> MAPITAYSQQTRGLLGCI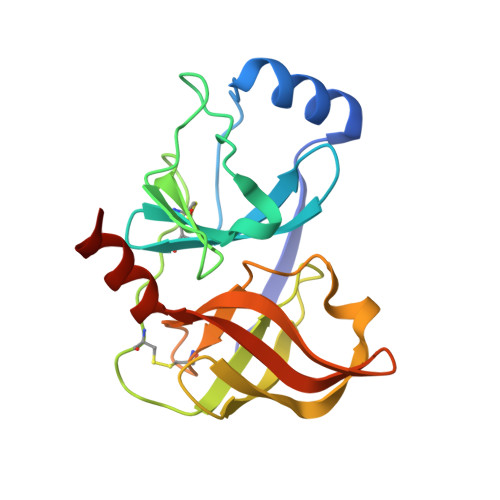ITSLTGRDKNQVDGEVQVLSTATQSFLATCVNGVCWTVYHGAGSKTLAGPKGPITQMYTNVDQDLVGWPAPPGARSMTPCTCGSSDLYLVTRHADVIPVRRRGDSRGSLLSPRPVSYLKGSSGGPLLCPSGHVVGIFRAAVCTRGVAKAVVFIPVESMETTMRASKKKK> MRPLTEEETRVMFEKIAKYIGENLQLLVDRPDGTYCFRLHNDRVYYVSEKIMKLAANISGDKLVSLGTCFGKFTKTHKFRLHVTALDYLAPYAKYKVWIKPGAEQSFLYGNHVLKSGLGRITENTSQYQGVVVYSMADIPLGFGVAAKSTQDCRKVDPMAIVVFHQADIGEYVRHEET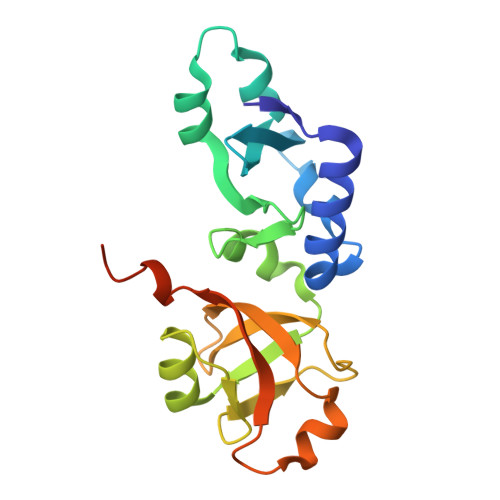LTLEHHHHHH>MLLYMRFTENFERAKKEALMSLEIALRKGEVDEDIIPLLKKINSIENYFTTSSCSGRISVMEMPHFGDKVNAKWLGKWHREVSLYEVLEAIKKHRSGQLWFLVRSPILHVGAKTLEDAVKLVNL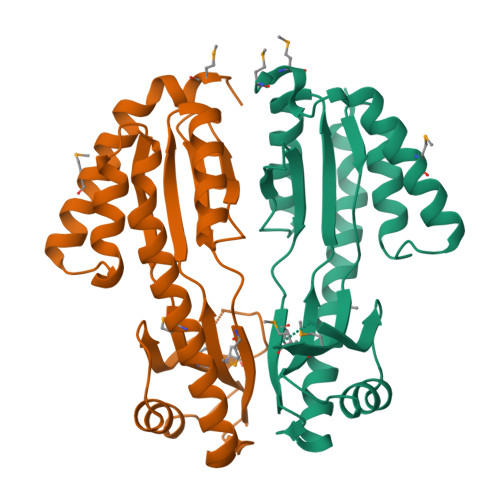AVSCGFKYSNIKSISNKKLIVEIRSTERMDVLLGENGEIFVGEEYLNKIVEIANDQMRRFKEKLKRLESKINALNR[2x]~{N}-[(4-ethylphenyl)methyl]-3-[5-[2-(1~{H}-indol-3-yl)ethyl]-1,3,4-oxadiazol-2-yl]-~{N}-methyl-propanamide | C25 H28 N4 O2 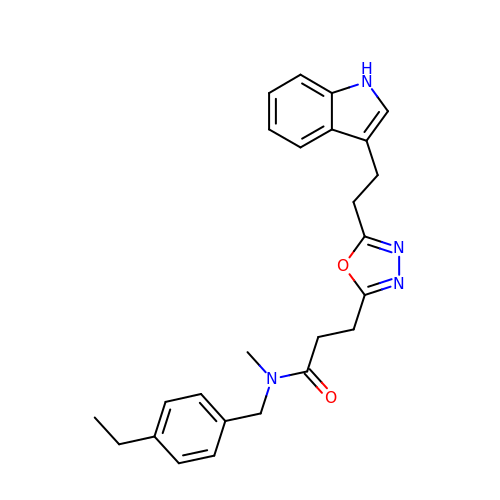| MYWFVOHKFIFWPL-UHFFFAOYSA-N> MKMVVAVIRPEKLECVKKALEERGFVGMTVTEVKGRGEQKGIRLQFRGREVEVDLLQKTKVEVVVSDDAVDEVVEAIVSSARTGKFGDGRIFVIPVEKSV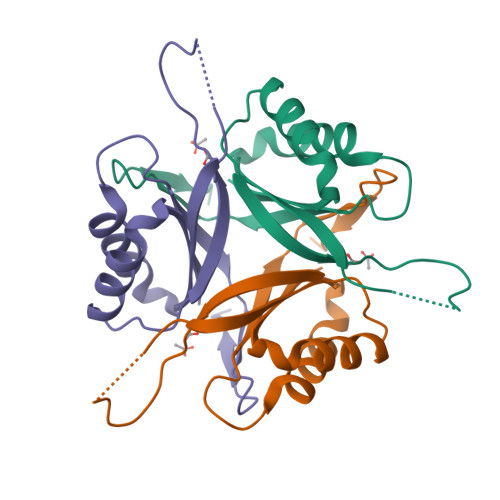KIRTGEEEVAAAHHHHHH(2R,4R)-1-cyclopropylcarbonyl-4-[[(2S,4S)-4-fluoranylpyrrolidin-2-yl]carbonylamino]-N-[[4-[2-[4-(morpholin-4-ylmethyl)phenyl]ethynyl]phenyl]methyl]pyrrolidine-2-carboxamide 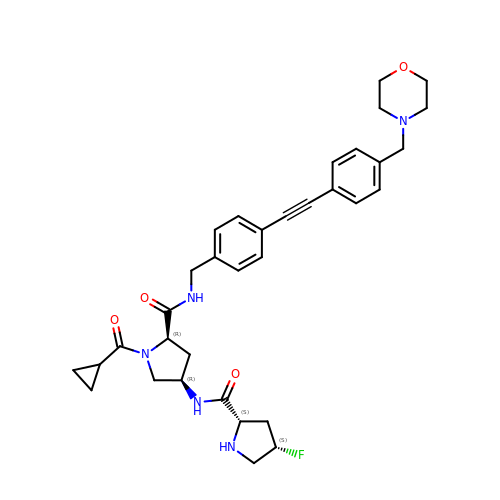| C34 H40 F N5 O4 | QHISDRDMHBJAEJ-XFBWMNOSSA-N>MQPMTARFDLFVVGSGFFGLTIAERVATQLDKRVLVLERRPHIGGNAYSEAEPQTGIEVHKYGAHLFHTSNKRVWDYVRQFTDFTDYRHRVFAMHNGQAYQFPMGLGLVSQFFGKYFTPEQARQLIAEQAAEIDTADAQNLEEKAISLIGRPLYEAFVKGYTAKQWQTDPKELPAANITRLPVRYTFDNRYFSDTYEGLPTDGYTAWLQNMAADHRIEVRLNTDWFDVRGQLRPGSPAAPVVYTGPLDRYFDYAEGRLGWRTLDFEVEVLPIGDFQGTAVMNYNDLDVPYTRIHEFRHFHPERDYRTDKTVIMREYSRFAEDDDEPYYPINT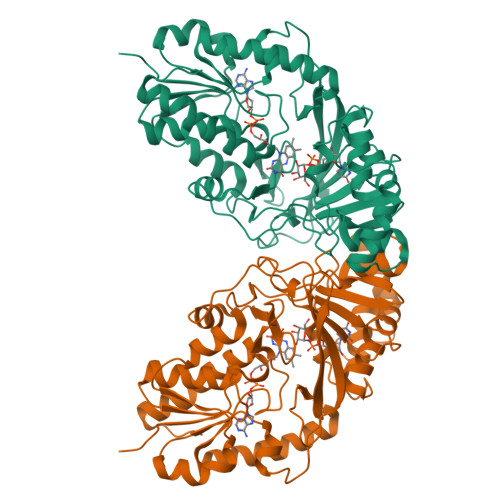EADRALLATYRARAKSETASSKVLFGGRLGTYQYLDMHMAIASALNMYDNVLAPHLRDGVPLLQDGA[3x]5-chloro-3-ethyl-N-{2-[4-(piperidin-1-yl)phenyl]ethyl}-1H-indole-2-carboxamide | C24 H28 Cl N3 O | 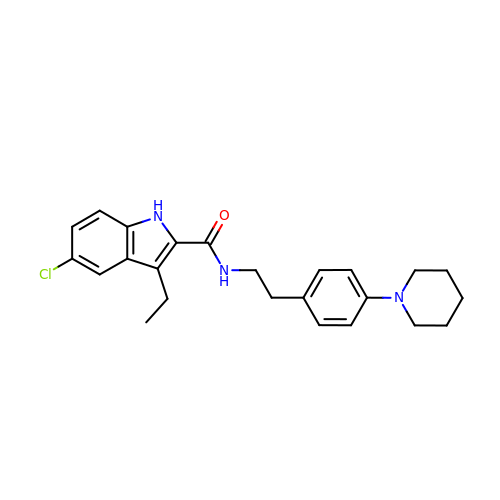AHFZDNYNXFMRFQ-UHFFFAOYSA-N> LPTDTTTFKRIFLKRMPSIRESLKERGVDMARLGPEWSQPMKRLTLGNTTSSVILTNYMDTQYYGEIGIGTPPQTFKVVFDTGSSNVWVPSSKCSRLYTACVYHKLFDASDSSSYKHNGTELTLRYSTGTVSGFLSQDIITVGGITVTQ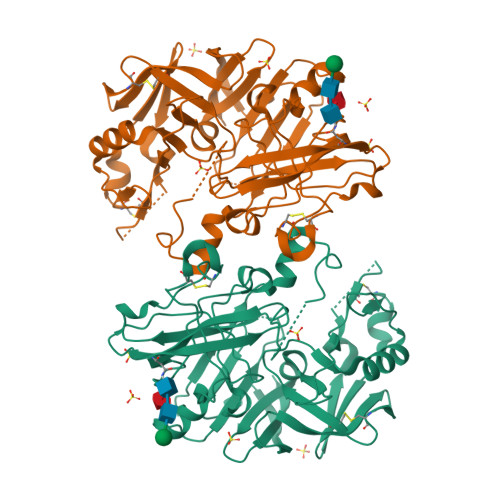MFGEVTEMPALPFMLAEFDGVVGMGFIEQAIGRVTPIFDNIISQGVLKEDVFSFYYNRDSENSQSLGGQIVLGGSDPQHYEGNFHYINLIKTGVWQIQMKGVSVGSSTLLCEDGCLALVDTGASYISGSTSSIEKLMEALGAKKRLFDYVVKCNEGPTLPDISFHLGGKEYTLTSADYVFQESYSSKKLCTLAIHAMDIPPPTGPTWALGATFIRKFYTEFDRRNNRIGFALAR> EFIEIVERSNYMGNPWTEYMAKYDIEEVHGSGIRVDLGEDAEVAGTQYRLPSGKCPVFGKGIIIENS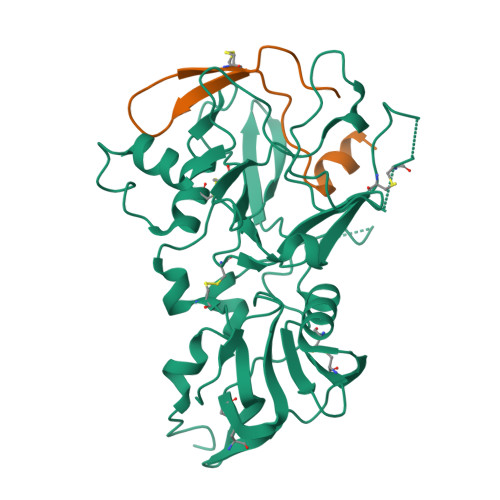KTTFLKPVATGNQDLKDGGFAFPPTNPLISPMTLNGMRDFYKNNEYVKNLDELTLCSRHAGNMNPDNDKNSNYKYPAVYDYNDKKCHILYIAAQENNGPRYCNKDQSKRNSMFCFRPAKDKLFENYVYLSKNVVDNWEEVCPRKNLENAKFGLWVDGNCEDIPHVNEFSANDLFECNKLVFELSASDQPKQYEQHLTDYEKIKEGFKNKNADMIKSAFLPTGAFKADRYKSHGKGYNWGNYNRETQKCEIFNVKPTCLINDKSYIATTALSHPIEVEHNFPGLEQKLISEEDLNSAVDHHHHHH;> MDISQHATDIGMGPATSCYTSTIPPPKQVCIQQAVKATL>SDAKETSATDLKRPREEDDNGGAATMETENGDQKKEPACFSTVIPGWFSEMSPMWPGEAHSLKVEKVLFQGKSDYQDVIVFQSATYGKVLVLDGVIQLTERDECAYQEMITHLPLCSIPNPKKVLVIGGGDGGVLREVARHASIEQIDMCEIDKMVVDVSKQFFPDVAIGYEDPRVNLVIGDGVAFLKNAAEGSYDAVIVDSSDPIGPAKELFEKPFFQSVARALRPGGVVCTQAESLWLHMDIIEDIVSNCREIFKGSVNYAWTSVPTYPSGVIGFMLCSTEGPDVDFKHPLNPIDESSS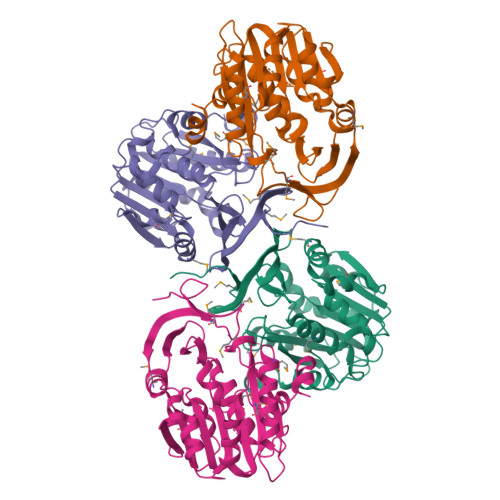KSNGPLKFYNAEIHSAAFCLPSFAKKVIESKAN[4x]> SQKVEKTVIKNETGTISISQLNKNVWVHTELGSFNGEAVPSNGLVLNTSKGLVLVDSSWDDKLTKELIEMVEKKFQKRVTDVIITHAHADRIGGIKTLKERGIKAHSTALTAELAKKNGYEEPLGDLQTVTNLKFGNMKVETFYPGKGHTEDNIVVWLPQYNILVGGCLVKSTSAKDLGNVADAYVNEWSTSIENVLKRYRNINAVVPGHGEVGDKGLLLHTLDLLK

Metallo-β-lactamases (MBLs) enable bacterial resistance to almost all classes of β-lactam antibiotics. There are two mechanistic types of β-lactamase – the serine β-lactamases (SBLs), which employ a nucleophilic serine (Ambler classes A, C, D) and the metallo-β-lactamases (MBLs), which utilise a Zn(II) bound hydroxide in β-lactam hydrolysis (class B). The enethiols inhibit MBLs from different subclasses. Crystallographic analyses reveal that the enethiol sulphur displaces the di-Zn(II) ion bridging ‘hydrolytic’ water.

The results reveal some SAR trends – some of the di-/tri-substituted amides and enethiols were clearly more active than the mono-substituted compounds. Thus, in most cases, the amides 5a-5e, showed almost no inhibition against all the subclass B1 MBLs (IC50 values ∼50 or >50 µM), when the para-position of the phenyl ring was mono-functionalised with halogen or alkyl groups. By contrast, e.g., the mono-ortho-substituted 5f-5i (IC50 values 2.0–52.1 µM), and di-ortho-substituted 5j (IC50 values < 2.0 µM), and 2,3,6-trifluoro 5k (IC50 values < 3.5 µM) analogues did manifest significant inhibition for all the tested B1 subclass MBLs, with the exception of NDM-1. Similar trends were observed for the enethiols 6a-6L, although IC50 values are mostly in the nanomolar range across all the MBLs tested. In each MBL the thiolate interacts with both Zn(II) ions and the inhibitor carboxylate interacts with Zn2 and (Lys-224 of BcII/Arg233 of VIM-2). The enethiol linked phenyl rings of the inhibitors all occupy the same region of the active site. As observed in the VIM-2:ML302F complex, the plane of the phenyl side chain on all of the enethiol inhibitors is rotated about the C3–C4 bond such that it is not co-planar with the plane of the enethiol alkene, likely hindering conjugation.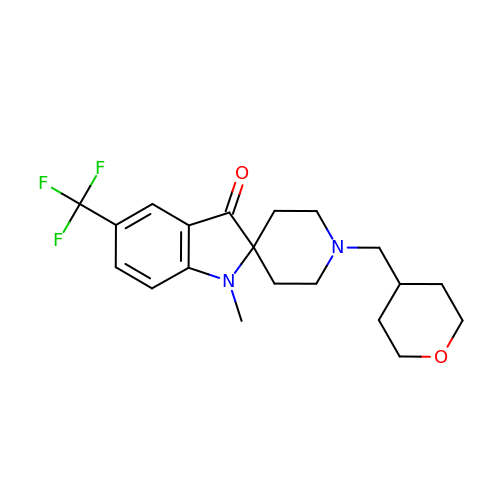1-methyl-1'-[(oxan-4-yl)methyl]-5-(trifluoromethyl)spiro[indole-2,4'-piperidin]-3(1H)-one | C20 H25 F3 N2 O2 | CEQWEVQYPPXCIW-UHFFFAOYSA-N The incorporation of amino acids into proteins is initiated by the 20 aminoacyl tRNA synthetases (AARSs). These enzymes attach each amino acid to its cognate tRNA, which is transferred to the ribosome to be used as building blocks for protein synthesis. Based on its molecular and structural similarity to alanine (Ala) and proline (Pro) (Aze has a 4- and Pro a 5-member ring), Aze is a dual mimic that might fit into the active site pocket of alanyl-tRNA synthetase (AlaRS) or prolyl-tRNA synthetase (ProRS) and be activated for protein synthesis. To establish whether Hs AlaRS and ProRS confuse Aze for Ala or Pro or both, we co-crystalized a stable analog of the aminoacyl adenylate of Aze (5′-O-[N-(L-azetidinyl) sulfamoyl] adenosine, Aze-SA) with both synthetases.

For all the experiments with Hs ProRS, recombinant protein corresponding to only the ProRS portion of the natural human glutamyl–prolyl–tRNA synthetase (GluProRS) fusion protein was used. Aze-SA fits into the active site of Hs ProRS in almost the same conformation as Pro-SA bound to Tt ProRS, showing that activated Aze is also a close mimic of Pro in the active site of Hs ProRS. Importantly, our co-crystal of Hs ProRS with the adenylate analog of Aze-AMP was closely similar to that of Tt ProRS in complex with the Pro-AMP analog. The dual mimicry of Aze, and its ability to ‘confuse’ two human tRNA synthetases, is established by these crystal structures. In a competition assay, we observed that Aze could efficiently compete with Pro for charging onto tRNAPro by Hs ProRS. Activation of Aze also resulted in significant production of Aze-tRNAPro. Consistent with an earlier report, Aze clearly escaped the editing function of Hs ProRS18. While Hs ProXp-ala hydrolyzes Ala-tRNAPro, it is unable to clear Aze-tRNAPro. Here we show that although Aze is activated by both human (Hs) AlaRS and Hs ProRS, it is rejected (>99%) by the AlaRS but not the ProRS editing system and therefore almost exclusively misincorporates into Pro positions of proteins. Surprisingly, while both Hs ProRS and Hs AlaRS activated Aze, only ProRS was successful in completing the charging event.

> MHHHHHHGSGEGQGPKKQTRLGLEAKKEENLADWYSQVITKSEMIEYHDISGCYILRPWAYAIWEAIKDFFDAEIKKLGVENCYFPMFVSQSALEKEKTHVADFAPEVAWVTRSGKTELAEPIAIRPTSETVMYPAYAKWVQSHRDLPIKLNQWCNVVRWEFKHPQPFLRTREFLWQEGHSAFATMEEAAEEVLQILDLYAQVYEELLAIPVVKGRKTEKEKFAGGDYTTTIEAFISASGRAIQGGTSHHLGQNFSKMFEIVFEDPKIPGEKQFAYQNSWGLTTRTIGVMTMVHGDNMGLVLPPRVACVQVVIIPCGITNALSEEDKEALIAKCNDYRRRLLSVNIRVRADLRDNYSPGWKFNHWELKGVPIRLEVGPRDMKSCQFVAVRRDTGEKLTVAENEAETKLQAILEDIQVTLFTRASEDLKTHMVVANTMEDFQKILDSGKIVQIPFCGEIDCEDWIKKTTARDQDLEPGAPSMGAKSLCIPFKPLCELQPGAKCVCGKNPAKYYTLFGRSY> SNAMISIPKDEFQQIFVKDLMISSEKVAHVQIGNGLEHALLVLVKSGYSAIPVLDPMYKLHGLISTAMILDGILGLERIEFERLEEMKVEQVMKQDIPVLKLEDSFAKALEMTIDHPFIC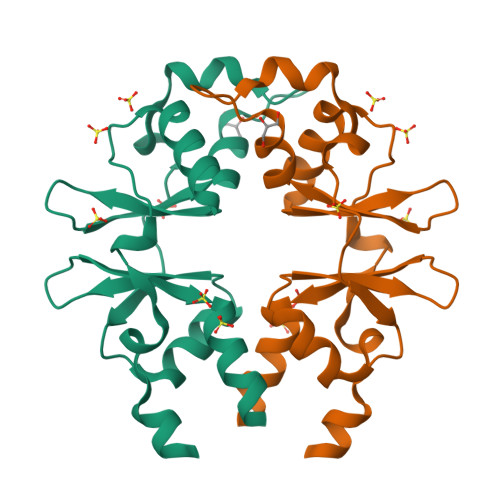AVNEDGYFEGILTRRAILKLLNKKVRQHNR> MVHAFLIHTLRAPNTEDTGLCRVLYSCVFGAEKSPDDPRPHGAERDRLLRKEQILAVARQVESMCRLQQQA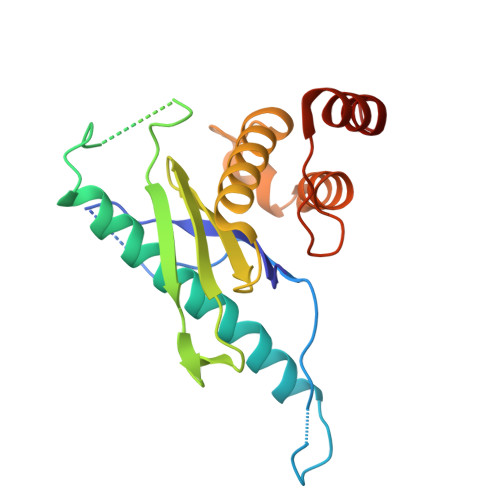SGRPPMDLQPQSSDEQVPLHEAPRGAFRLAAENPFQEPRTVVWLGVLSLGFALVLDAHENLLLAEGTLRLLTRLLLDHLRLLAPSTSLLLRADRIEGILTRFLPHGQLLFLNDQFVQGLEKEFSAAWPR> ASVHGTTYELLRRQGIDTVFGNPGSNELPFLKDFPEDFRYILALQEACVVGIADGYAQASRKPAFINLHSAAGTGNAMGALSNAWNSHSPLIVTAGQQTRAMIGVEALLTNVDAANLPRPLVKWSYEPASAAEVPHAMSRAIHMASMAPQGPVYLSVPYDDWDKDADPQSHHLFDRHVSSSVRLNDQDLDILVKALNSASNPAIVLGPDVDAANANADCVMLAERLKA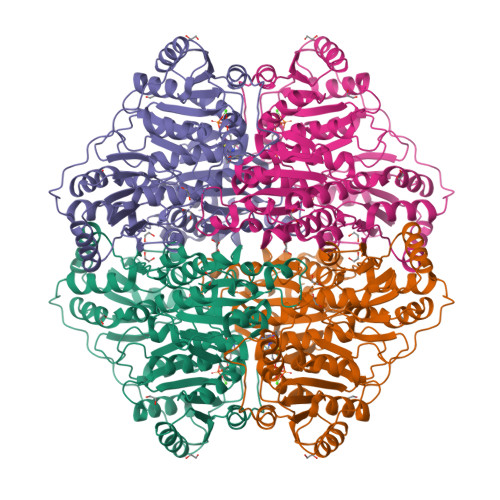PVWVAPSAPRCPFPTRHPCFRGLMPAGIAAISQLLEGHDVVLVIGAPVFRYTQYDPGQYLKPGTRLISVTCDPLEAARAPMGDAIVADIGAMASALANLVEESSRQLPTAAPEPAKVDQDAGRLHPETVFDTLNDMAPENAIYLNESTSTTAQMWQRLNMRNPGSYYFCAAGGLGFALPAAIGVQLAEPERQVIAVIGDGSANYSISALWTAAQYNIPTIFVIMNNGTYGALRWFAGVLEAENVPGLDVPGIDFRALAKGYGVQALKADNLEQLKGSLQEALSAKGPVLIEVSTVSPHHHHHH> MTRLLVLGGTTEASRLAKQDADQGFEAVFSYAGRTGAPVAQPLPTRIGGFGGVAGLVDYLTREGVSHVIDATHPFAAQMSANAVAACAQTGVALCAFERAPWTAQAGDRWTHVPDLAAAVAALPQAPARVFLAIGKQHLRDFSAAPQHHYLLRLVDPPEGPLPVPDARAVIARGPFTVQGDTELLRSETITHVVAKNAGGAGAEAKLIAARSLGLPVILIDRPAVPARDICATLEGVMGWLADHGATPRGV

In this paper we investigate the structure of the precorrin-6A reductase CobK involved in the aerobic pathway, there is a homologous enzyme CbiJ involved in the anaerobic pathway both enzymes catalyse the NADPH-dependent reduction of precorrin-6A5 to the dihydro derivative precorrin-6B6. We have determined the structure of apoenzyme, holoenzyme and a ternary complex with NADPH and product giving unprecedented insights into the structure and mechanism of CobK. CobK comprises two domains, a coenzyme binding domain and a substrate-binding domain, both of β/α architecture. CobK unusually comprises two parallel β-sheet domains arranged so the β-strands point towards the centre of the molecule where the NADPH and substrate bind.

The apoenzyme and holoenzyme structures at 3.17 Å and 1.63 Å respectively lack the β2/β3 loop which is disordered and the apoenzyme structure is less well defined overall than the binary and ternary complexes. The N- and C-terminal domains have a relatively small contact surface, there is only 304 Å2 of solvent accessible surface buried between the two domains in the apoenzyme and only two connections both comprising irregular polypeptide chain; therefore there is considerable opportunity for the domains to move with respect to one another. The presence of coenzyme, which buries 361 Å2, limits this movement and the presence of precorrin product provides further rigidity. The picture therefore is one of increasing rigidity of the structure as first NADPH and then precorrin binds. The CobK apoenzyme has few contacts between the coenzyme and substrate binding domains; the structure becomes increasingly rigid as first coenzyme binds and then product and this is reflected in the resolution to which the respective crystals diffracted.4-{1-[2-(4-methyl-1H-1,2,3-triazol-1-yl)ethyl]-4-phenyl-1H-imidazol-5-yl}benzonitrile | C21 H18 N6 | 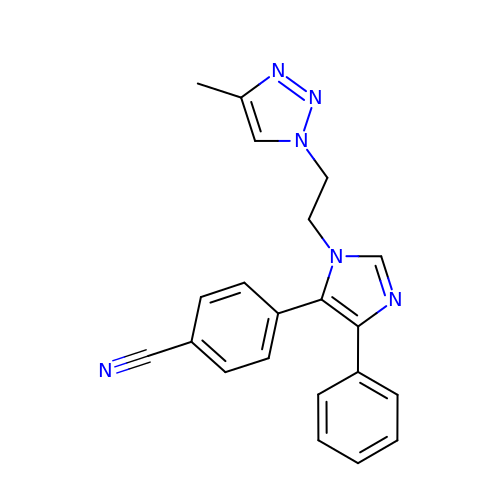OAPIWVHFYSEARE-UHFFFAOYSA-N> ETGSVSKTEHAEINIFSVASGHLYERMLNIMMASVMHHTNHTVKFWFIEQFLSPSFKDFIPHMAAEYGFKYEMVTYKWPHWLRQQKEKQREIWGYKILFLDVLFPLSLDKVIFVDADQIVRTDMYDLVEHPLDGAPYGFAPMCDSRVEMEGYRFWKTGYWANYLKGKPYHISALYVVDLQRFRELAAGDRLRQQYHALSADPNSLANLDQDLPNHMQFTIPIATLPQEWLWCETWCSDETLKDARTIDLCNNPMTKEPKLDRARRQVPEWTKYDEEIAELARRVREGTKHHHHHH

For example, the envelope glycoproteins of many viruses are exquisitely dependent on calnexin-mediated folding, a process enabled by the action of the ER endoplasmic reticulum enzyme UDP–Glc glycoprotein glucosyltransferase (UGGT) and the ER alpha glucosidases I and II. ER alpha glucosidases I and II usher client proteins in and out of the calnexin cycle, which is part of the glycoprotein folding quality control in the ER, whilst UGGT plays a key role in retaining misfolded glycoproteins in the ER for a “second chance” at folding correctly. We could not crystallise the GT24 catalytic domain of human UGGT—so we used crystals of the GT24 catalytic domain of CtUGGT (hereinafter CtUGGT GT24) instead. The sequence of this fungal UGGT has about 70% similarity and 60% identity to the ones of the same domain of the two human UGGT isoforms (UGGT1 and UGGT2) so that any ligands found with the crystals of CtUGGT would likely bind the human enzymes too—paving the way to a medicinal chemistry program towards modulators of human UGGT activity.

In the course of an X-ray crystallography FBLD effort aimed at the discovery of molecules binding the catalytic domain of Chaetomium thermophilum UGGT (CtUGGT GT24), we encountered crystal polymorphism: the majority of CtUGGT GT24  crystals belonged to space group H3, but some crystals lowered their symmetry to an equivalent P1 pseudo-rhombohedral lattice. The best hit was a CtUGGT GT24  2.2 Å  H3 crystal soaked in 5M-8OH-Q. The molecule is bound to a conserved patch on the surface of the protein. Diffraction data from this crystal process in H3 with Rmeas H3 = 0.323 and in P1 with Rmeas P1 = 0.206. The CCP4-Dimple/REFMAC5 Rfrees are Rfree H3 = 0.227 and Rfree P1 = 0.2537. The compound binds to a conserved patch on the surface of the CtUGGT GT24  domain, about 15 Å  away from the UDP–Glc binding site. The morpholine ring is partially disordered in the crystal, but one of its ring placements is 4.2 Å  from the conserved 1396DQD1398 motif coordinating the Glc ring of UDP–Glc; the ligand also causes a displacement of the side chain of CtUGGT GT24  1346Y. Through this displacement, the 8OH-quinoline ring inserts and is sandwiched between the aromatic side chains of the conserved residues 1346YW1347—which we propose to call the “YW clamp. The two aromatic side chains stabilise the quinoline ring, forming an aromatic trimer; the 8-OH group of the quinoline also establishes an H-bond to the side chain of 1402H. The compound is now the starting point for a medicinal chemistry programme that will develop more potent and selective UGGT inhibitors.>[2x]MSAYDSGKT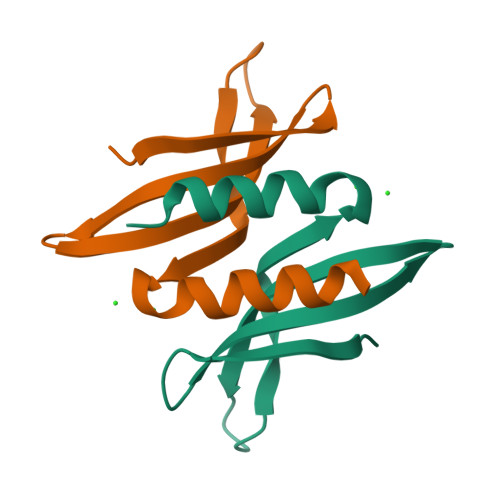IADVQKSATQRIRISHRWYRGRRYVDVRLVVVDRDGDFVPTRQGISIRPELLAQVIQGLLLASREG>[2x]GAMDPSSPNYDKWEMERTDITMKHKLGGGQYGEVYEGVWKKYSLTVAVKTLKEDTMEVEEFLKEAAVMKEIKHPNLVQLLGVCTREPPFYIITEFMTYGNLLDYLRECNRQEVSAVVLLYMATQISSAMEY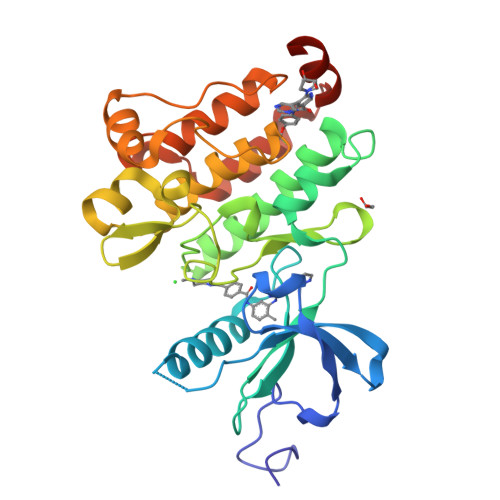LEKKNFIHRDLAARNCLVGENHLVKVADFGLSRLMTGDTYTAHAGAKFPIKWTAPESLAYNKFSIKSDVWAFGVLLWEIATYGMSPYPGIDLSQVYELLEKDYRMERPEGCPEKVYELMRACWQWNPSDRPSFAEIHQAFETMFQESSISDEVEKELGKRGT> GHMGLFGKTQEKPPKELVNEWSLKIRKEMRVVDRQIRDIQREEEKVKRSVKDAAKKGQKDVCIVLAKEMIRSRKAVSKLYASKAHMNSVLMGMKNQLAV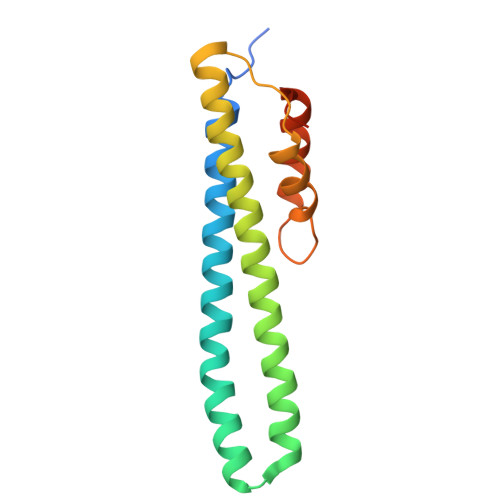LRVAGSLQKSTEVMKAMQSLVKIPEIQATMRELSKEMMKAGIIEEMLEDTFES> P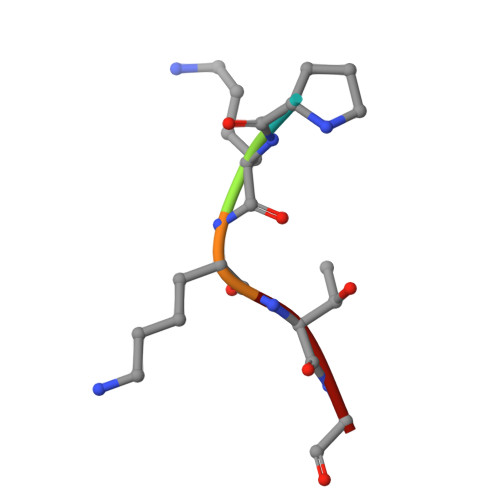KKTG> MIDLRLEEDILTATLPEFLSTRPKYRYAYTNTKQQDIRFQGPMRHVRLTHLYKQTKLWNLQYIERELAISEIDDALDEFIQTFSLPYVIEQGTYKYNMLLGMHAHNVNYQDDVSELIANNPQLLNYLDDNPFSAIFELVNVDLQIYQYGQNIFNNEAEHTILFLKDNTNYGVIQALQKHPFSATHINWHLHKHIFVFHSREQLLNKLLSAGLEDSQLYQRQKTYSTKRGDRPTERMV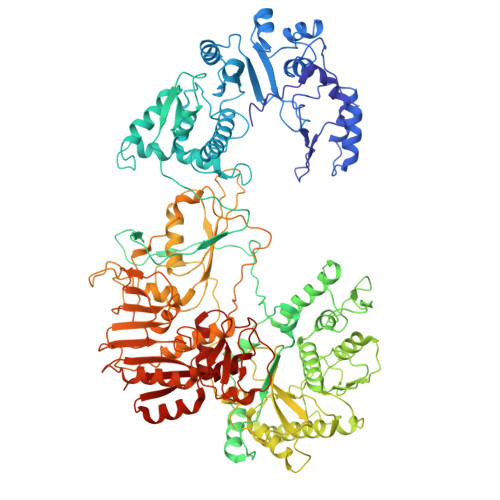TYIEDDHIRRIQAVFPLLLDNIFDVKLHKDSSMTWLKSYADMIYDSVKNSNSTITPEIRKLYLRMYNQYMRIFLPIEQYMLYDNTCWPFSEKITLKINVRLISSRENQPVLWKTPIDTENLISIVQPDEPINKLNFTAIPSTMIRLNDNITMYRAVKDMFSAIEYLPDAIENIPTLTMKEQALSRYISPDSEAQNFFNNQPPYLNSIMNVNRQVFEAVKRGNIQVSTGSMEHLCLCMHVKSGLIVGRTVLIDDKVVLRRNFNASTAKMITCYVKAFAQLYGEGSLINPGLRMVFFGVETEPAIDILKLFYGDKSLYIQGFGDRGIGRDKFRTKIEDALTLRIGCDILISDIDQADYEDPNEEKFDDITDFVCYVTELVISNATVGLVKISMPTYYIMNKISSTLNNKFSNVAINIVKLSTQKPYTYEAYIMLSHGSTLTNKGYLRNPVCDVYLEKISLQPMDLKIISTISNEINYDKPTLYRFVVDKNDVTDVSIAMHILSIHCSTITTRSVMVRSDNTGAFVTMSGIKDMKRVAIMNRMTDGTSANSYMHEQNGKLYLQKVPYLEDLISAFPNGFGSTYQNDYDSSMSVINVNALIRQVVYRVISKSIPVALLESLSRIRIIGGRDLGEMNAVYKLYKTPIEVYDAVGITREYPHVQISYRAQRYSFTESIPNHTLLLANYVIMNDVDGAPISSLEQINTIKKIISKISLGSIAYIQVYTDIVARNINVMTKNDSFLISANADKTVFKVQVSGYKAVEMCNYEQLLQLVSDNTGVNIIKLTYQDVLESCVLSSGILGDTGSWLLDLVLASTYIIEIRG>MSASDGQGMRAVILVGGFGTRLRPLTLTTPKPLVPFCNKPMIIHQIEALKAVGVTEVILAVAYRPEAMKEQMDEWSRKLGVSFVFSVEEEPLGTAGPLALARDILMQDDKPFFVLNSDVTCTFPMQELLDFHKAHGGEGTIMVSQVTQWEKYGVVVYSPQNYQIERFVEKPSRFLGDRINAGIYIFNKSILDRIPPRRASIEKEIFPAMAAEGQLYAFNLEGFWMDVGQPKDYILGMTKFIPSLVHGNRETEQLHTEAVEHQRGGRFTVIGASLIDPSAKIGDGAVIGPYASIGANCVIGESCRIDNAAILENSKVGKGTMVSRSIVGWNNRIGSWCHIKDISVLGDDVEVKDGVILIGTKVLPNKDVGEHRFEPGIIM[6x]

A prominent therapeutic target for antileishmanial drug development is leishmanial GDP-mannose pyrophosphorylase (GDP-MP or GMPP, EC 2.7.7.13), an enzyme catalyzing the formation of GDP-mannose by condensation of mannose-1-phosphate (Man-1-P) and GTP. As GDP-mannose serves as a central precursor for biosynthesis of diverse glycoconjugates necessary for host–parasite recognition and is essential for parasite survival, disruption of Leishmania GDP-MP activity leads to complete loss of virulence, suggesting this enzyme as an attractive target for development of new drugs against leishmaniasis. LdGDP-MP exhibits a hexameric structure with a molecular weight of ~245.3 kDa, consistent with previous observations. Each subunit is made of two separate domains, a N-terminal Rossmann-like fold commonly observed in nucleotidyltransferases and many other nucleotide-binding proteins, and a C-terminal left-handed β-helix domain containing tandem repeats of a [I/L/V]-G-X(4) hexapeptide motif, a characteristic structure found in the transferase hexapeptide repeat family.

To gain insights into the catalytic mechanism of leishmanial GDP-MP, we further solved the cryo-EM structures of LdGDP-MP in complex with its substrate, GTP, or the reaction product, GDP-mannose at the resolution of 3.0 Å, or 3.2 Å, respectively. These structures clearly mark a closed and well-ordered active pocket with approximate dimensions of 14 Å × 15 Å × 17 Å, delimited by β1–β4–β9 in the central β-sheets as the pocket base. Structural comparisons reveal that binding to GTP or GDP-mannose induces significant conformational changes primarily for the loop regions surrounding the active site, and results in an overall more compact conformation. Indeed, the key lysine residue (K170) in the F(V)EKP motif shifts ~5 Å or ~8 Å towards the catalytic center upon GTP or GDP-mannose binding. In the GDP-mannose-bound LdGDP-MP, the guanidine moiety, compared to that in the GTP-bound form, scrunches ~4 Å from the cleft end towards the catalysis center. Intriguingly, the GDP-mannose molecule adopts a seemingly unfavorable V-shape conformation, which may facilitate the condensation reaction and subsequent product release. The sugar moiety is secured by the close contact of the hydroxyls with the central β-sheet amino acids, as well as the Mg2+-coordinating residue D226. In particular, the K170 side-chain in the F(V)EKP motif inserts deeply into the catalytic center to make close contact with the phosphate group next to the sugar moiety, indicative of its direct involvement in catalysis. The catalytically essential Mg2+ is coordinated by two absolutely conserved aspartate residues, D118 and D226.N-{3-[(2R)-6-{[3-amino-4-(morpholine-4-carbonyl)phenyl]amino}-5-oxo-2,5-dihydropyrazin-2-yl]-2-methylphenyl}-4-(piperidin-1-yl)benzamide 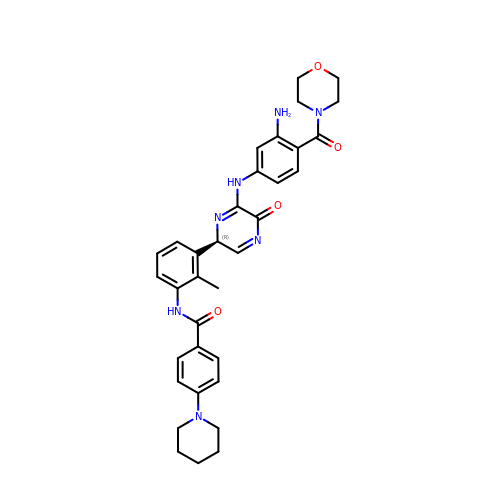| C34 H37 N7 O4 | DCSDBJGDUKAXOF-UHFFFAOYSA-N> GSAKDPMQIVSINVGKPKTIEVNGERLVTGIDKTPVAHPVAVGKQNLAGDGQADLVHHGGEDKAICAYPSEHFVYWEERYGRPFTAGAFGENWTLLGLTEDDVCLGDIYVAGTALVQVSQPRQPCSKLAFKHQLPDLPKAICQTGKSGFYFRVLQEGVIEPGAPLVLVERGVGALSIAYINHIYYHERDNAAAMKQIASHPALSASWRETFQKRLADRPRP

MOSC proteins play a key role in the Moco-dependent reduction of N-hydroxylated mutagens or prodrugs as a final electron transfer enzyme in the nitrogen-reducing system. To provide insights into the catalytic mechanism of MOSC enzymes, we report two crystal structures of YiiM, one from Gram-positive Geobacillus stearothermophilus (gsYiiM) and the other from Gram-negative E. coli (ecYiiM). Based on the comparative analyses of structural and biophysical data, we present the common and distinct features of YiiM enzymes and propose the putative catalytic site that is located at a reactive invariant cysteine residue. Sequences corresponding to the β-barrel and N-α-bundle modules of YiiM are conserved in MOSC family members, suggesting that the two modules form the canonical structure of the MOSC domain.

The crystal structure of gsYiiM was determined by molecular replacement and refined to 2.00 Å resolution. The gsYiiM structure consists of ten β-strands and six α-helices and folds into a triangular shape that can be divided into three distinct structural modules, namely, a β-barrel, an N-terminal α-helix bundle (N-α-bundle), and a C-terminal α-helix bundle (C-α-bundle). gsYiiM possesses a cavity in the middle of its triangular architecture. The gsYiiM cavity holds an invariant cysteine residue (C119 in gsYiiM), which is absolutely conserved in the entire MOSC family. Unexpectedly, in the Fo-Fc electron density map of gsYiiM, the sulfur atom of C119 exhibited an atypical triangular shape rather than a regular spherical shape that was observed for those of the other three cysteine residues (C60, C98, and C136) of gsYiiM. Considering the unusual shape and size of the electron density, the C119 sulfur atom is highly likely to have been oxidized to a sulfonic acid. Thus, the C119 residue was built in the gsYiiM structure as a cysteine sulfonic acid with good refinement statistics. The positive electrostatic potentials that surround the C119 residue would lower the pKa value of the sulfhydryl group at C119, and the deprotonated sulfur could readily make a nucleophilic attack on Moco for cofactor conjugation or on a substrate for the nitrogen-reducing process. Additionally, gsYiiM was observed as a monomer in the asymmetric unit without any suggestive oligomerization partner. In contrast, the α5-α6 loop of gsYiiM protrudes and makes significant steric clashes with the α5ʹ-α6ʹ loop in the dimeric organization, providing an explanation why gsYiiM prefers a monomeric form although the dimerization interface residues of ecYiiM are largely conserved in gsYiiM.>MQQLNENKIIKLLRDNIPKLQLIYLFGSYSQGTQHRNSDIDIAVLAADTLDNIARWELAQKLASALDSDVDLVDLRSASTVLCQQVVTQGKQLWGTQQDDELFAVKTISMYQHLQAERQAIIDDVMANTAAKAHRGESL[2x];>MNDIIINKIATIKRCIKRIQQVYGDGSQFKQDFTLQDSVILNLQRCCEACIDIANHINRQQQLGIPQSSRDSFTLLAQNNLITQPLSDNLKKMVGLRNIAVHDAQELNLDIVVHVVQHHLEDFEQFIDVIKAE[6x]

Our subsequent work demonstrated that the HEPN protein with a RX4–6H motif is the toxin which cleaves mRNA in vitro in the HEPN/MNT (SO_3166/SO_3165) TA pair in the model psychrotrophic bacterium Shewanella oneidensis. Furthermore, antitoxin SO_3165 binds to toxin SO_3166 at a rare 2:6 ratio to form a hetero-octamer, and this binding is important for the antitoxin to block the toxicity of the toxin. Specifically, structural and biochemical studies of the HepT/MntA TA pair (SO_3166/SO_3165) in S. oneidensis show that the GSX10DXD motif of antitoxin MntA is responsible for transferring three AMPs to HepT and that Y104 in RX4HXY in HepT is the site that receives three AMPs from MntA. We found here that MntA antitoxin acts as an adenylyltransferase and catalyzes the transfer of three AMP moieties onto toxin HepT to block its toxicity, representing a new type of interaction between the toxin and the antitoxin.

The results clearly show that substitution of the Y104 residue of HepT prevents adenylylation by MntA. We determined the crystal structures of HepT/MntA and HepTY104A/MntA at 3.08 and 2.6 Å, respectively. Similarly, a (HepT)6-(MntA)2 hetero-octamer was found in the ASU of HepTY104A/MntA. In contrast, this additional electron density map was no longer present in the HepTY104A/MntA complex. Comparison of the polyadenylylated HepT and unmodified HepTY104A revealed that they were nearly identical with an RMSD of 0.396 Å over the 953 Cα main chain, except for the loop containing Y104, which was rotated clockwise nearly 180°. The MntA molecule in HepT/MntA was almost identical to its counterpart in HepTY104A/MntA, with a maximal root mean square deviation (RMSD) of 0.26 Å over 98 Cα and 0.29396 Cα, respectively. Although substitution of Y104 in the RX4HXY motif did not affect the toxicity of HepT, this substitution clearly reduced the ability of MntA to neutralize HepT.> MSKVDLWQDATAQAELVRSGEISRTELLEATIAHVQAVNPEINAVIIPLFEKARRESELASGPFAGVPYLLKDLTVVSQGDINTSSIKGMKESGYRADHDAYFVQRMRAAGFVLLGKTNTPEMGNQVTTEPEAWGATRNPWNLGRSVGGSSGGSGAAVAAALSPVAHGNDAAGAVRIPASVCGVVGLKPTRGRISPGPLVTDSDNVAGAAHEGLFARSVRDIAALLDVVSGHRPGDTFCAP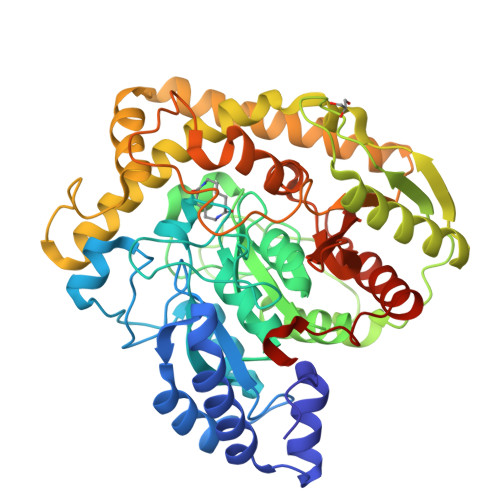TASRPYAQGISENPGSLRVGVLTHNPVGDFALDPECAAAARGAAAALAALGHDVNDAYPEALGDRSFLKDYSTICDVAIAREIERNGELIGRPLTEDDVEWTSWEMVKRADQVTGRAFAACVDELRYYAGKVERWWEAGWDLLILPTVTRQTPEIGELMLAKGTDLEGRQSAFISGSLQMLAFTVPFNVSGQPAISLPIGMSSDGMPIGVQIVAAYGREDLLLQVAAQLEGALPWVARRPQLLNPSRKIPAA> MMDAFEKVRTKLETQPQEEYEIINVEVKHGGFVYYQEGCCLVRSKDEEADNDNYEVLFNLEELKLDQPFIDCIRVAPDEKYVAAKIRTEDSEASTCVIIKLSDQPVMEAS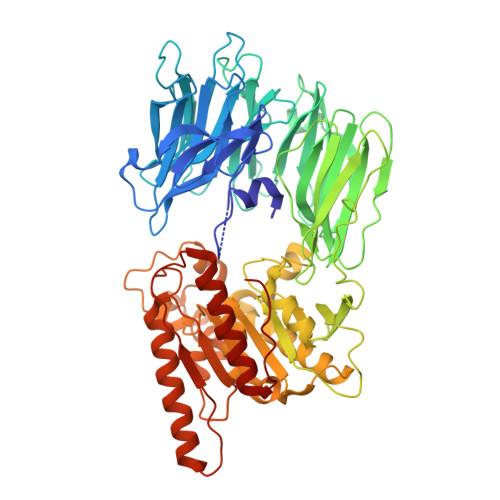FPNVSSFEWVKDEEDEDVLFYTFQRNLRCHDVYRATFGDNKRNERFYTEKDPSYFVFLYLTKDSRFLTINIMNKTTSEVWLIDGLSPWDPPVLIQKRIHGVLYYVEHRDDELYILTNVGEPTEFKLMRTAADTPAIMNWDLFFTMKRNTKVIDLDMFKDHCVLFLKHSNLLYVNVIGLADDSVRSLKLPPWACGFIMDTNSDPKNCPFQLCSPIRPPKYYTYKFAEGKLFEETGHEDPITKTSRVLRLEAKSKDGKLVPMTVFHKTDSEDLQKKPLLVHVYGAYGMDLKMNFRPERRVLVDDGWILAYCHVRGGGELGLQWHADGRLTKKLNGLADLEACIKTLHGQGFSQPSLTTLTAFSAGGVLAGALCNSNPELVRAVTLEAPFLDVLNTMMDTTLPLTLEELEEWGNPSSDEKHKNYIKRYCPYQNIKPQHYPSIHITAYENDERVPLKGIVSYTEKLKEAIAEHAKDTGEGYQTPNIILDIQPGGNHVIEDSHKKITAQIKFLYEELGLDSTSVFEDLKKYLKF2,4,6,8-tetrahydroxy-1,3,5,7,2lambda~5~,4lambda~5~,6lambda~5~,8lambda~5~-tetroxatetraphosphocane-2,4,6,8-tetrone 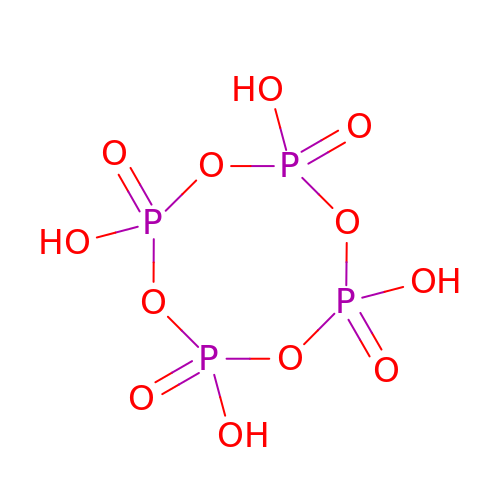| H4 O12 P4 | GIXFALHDORQSOQ-UHFFFAOYSA-N Ricin toxin is a potent ribosome-inactivating protein derived from the castor bean and a relatively common bioterrorism agent. The heterodimeric toxin consists of a lectin B-chain linked by a disulfide bond to a catalytic A-chain (RTA). Free RTA inside the cell can irreversibly inactivate ribosomes by cleaving the glysosidic bond of a specific adenine base in the sarcin/ricin domain of 28S ribosomal RNA. RTA has a single tryptophan, residue 211, located at the active site pocket.

However, we found that the position of Tyr80 in a newly determined structure of RTA soaked in 2 mM adenine was not the same as that previously reported. The electron densities of the ring and Cα-Cβ-Cγ bonds were clear throughout refinement, indicating re-orientation of the side-chain to the relatively common t80° rotamer. In this position, the hydroxyl group of Tyr80 can hydrogen bond with the amide nitrogen of Gly121. Upon examination of a crystal complex of RTA with adenine formed by soaking with adenine instead of AMP, we found that the overlap of the tyrosine 80 ring with the purine was much less than previously reported, due to a difference in side-chain rotameric position. The RTA-urea and RTA-adenine complexes also showed similar fluorescence spectra and a splayed arrangement of Arg180, while the positions of Tyr80 in these complexes differed. The orientation of Tyr80 did not therefore appear to control the fluorescence emission of Trp211. Watanabe et al. found that binding of adenine to the RTA depurination site as monitored by fluorescence had a KD of 1 mM, in agreement with our figure of 0.7 ± 0.05 mM. For the larger and tighter-binding ligand adenine, ΔH° was -53 kJ/mol (R = 0.97) with a ΔS° of -0.12 ± 0.01 kJ/(K*mol).

> MIFPKQYPIINFTTAGATVQSYTNFIRAVRGRLTTGADVRHEIPVLPNRVGLPINQRFILVELSNHAELSVTLALDVTNAYVVGYRAGNSAYFFHPDNQEDAEAITHLFTDVQNRYTFAFGGNYDRLEQLAGNLRENIELGNGPLEEAISALYYYSTGGTQLPTLARSFIICIQMISEAARFQYIEGEMRTRIRYNRRSAPDPSVITLENSWGRLSTAIQESNQGAFASPIQLQRRNGSKFSVYDVSILIPIIALMVYRCAPPPSSQF> AGAGGAGAUCUUCUCU

To further understand the structure and properties of the D:U base pair and the D:C mismatch, we designed and synthesized self-complementary RNA sequences that form duplexes with two separated or adjacent D:U or D:C pairs. All four oligonucleotides crystallized within 2–3 days at 20 °C under their optimal crystallization conditions, and we solved their structures by X-ray diffraction at a resolution higher than 1.65 Å. We found that all four structures adopt the same space group (R32). Each unit cell contains only a single RNA strand so that each duplex features two identical D-containing base pairs.

The sequence UD-1, 5′-AGA GDA GAU CUU CUC U-3′, can form two separated D:U pairs with the underlined nucleobases, while the sequence CD-1, 5′-AGA GDA GAU CUC CUC U-3′, can form two separated D:C pairs. Our crystallographic studies show that the D:U base pair has the expected Watson–Crick geometry. Whether separated (UD-1) or adjacent (UD-2) within the RNA duplex, the D:U pairs have identical geometries and exhibit three hydrogen bonds. Relative to a canonical A:U base pair, the third hydrogen bond is between the exocyclic 2-amino group and O2 of U. The H-bond distances between N6–O4, N1–N3, and N2–O2 in both D:U pairs are identical: 2.8, 2.9, and 2.8 Å, respectively. In RNA duplexes, D forms three hydrogen bonds when paired with U, as opposed to two in the A:U pair. This, together with a stronger stacking interaction, results in a D:U base pair being energetically more favorable than an A:U base pair. The larger degree of stabilization is also evidenced by a significant rise in the experimentally determined melting temperature (Tm) of D:U RNA duplexes compared to A:U duplexes. As a result, we observed a 20-fold increase in the binding of the substrate (D*D vs A*A) to a −UU– template.>MGPLPRTVELFYDVLSPYSWLGFEILCRYQNIWNINLQLRPSLITGIMKDSGNKPPGLLPRKGLYMANDLKLLRHHLQIPIHFPKDFLSVMLEKGSLSAMRFLTAVNLEHPEMLEKASRELWMRVWSRNEDITEPQSILAAAEKAGMSAEQAQGL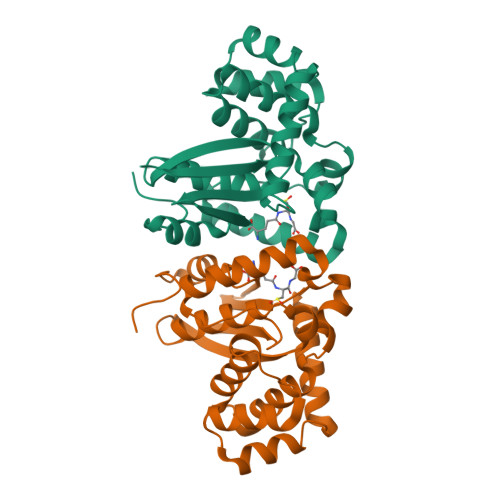LEKIATPKVKNQLKETTEAACRYGAFGLPITVAHVDGQTHMLFGSDRMELLAHLLGEKWMGPIPPAVNARL[2x]> SNATDGGWTPQRAANRLVKVVEAVSVAHGIDRFPVDVPQLALECAHIFKWPDPITKVQAAAIKGFDGALFAGESRKEWLLLYNDAVTSPGRMRFTQAHELGHYILHRMQRESFQCSDADMLNWSQDERDIEAQADLFASYLLMPLDDYRKQVTTDVDMDILGACAERY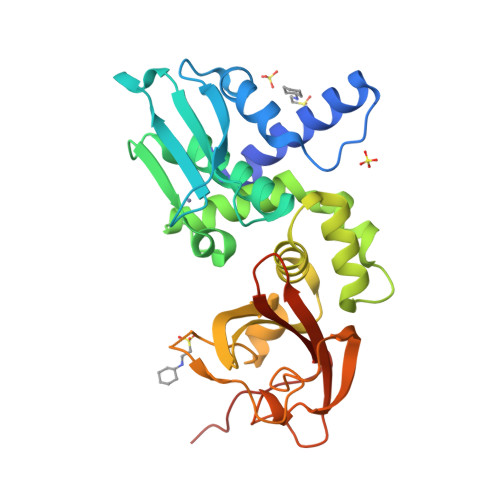GVSLTAAVLKWLQYTDEKAVLVMSNDGFINWAWSSEPAARAGAFFRTRGNVIPLPEGSLAANPEILHDRHGTKIPATVWFPHADPHIPLREMKIHAAQYDATLSLLWLPRSAEVWPPRERLEG> GTDVKNNEDYKNVDYKNVNFLQYHFKELSNYNIANSIDILQEKEGHLDFVIIPHYTFLDYYKHLSYNSIYHKSSTYGKCIAVDAFIKKINETYDKVKSKCNDIKNDLIATIKKLEHPYDINNKNDDSYRYDISEEIDDKSEETDDETEEVEDSIQDTDSNHTPSNKKKND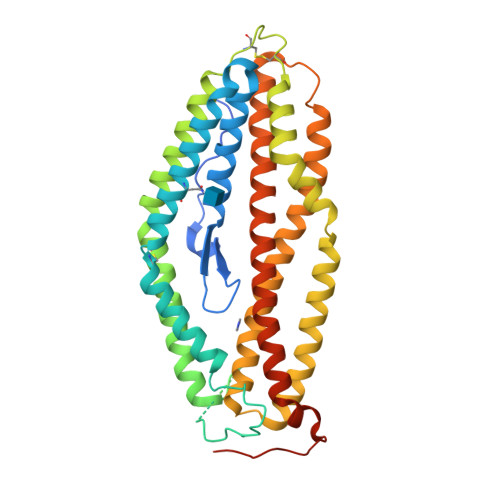LMNRTFKKMMDEYNTKKKKLIKCIKNHENDFNKICMDMKNYGTNLFEQLSCYNNNFCNTNGIRYHYDEYIHKLILSVKSKNLNKDLSDMTNILQQSELLLTNLNKKMGSYIYIDTIKFIHKEMKHIFNRIEYHTKIINDKTKIIQDKIKLNIWRTFQKDELLKRILDMSNEYSLFITSDHLRQMLYNTFYSKEKHLNNIFHHLIYVLQMKFNDVPIKMEYFQTYKKNKPLTQ S-(2-CARBOXY-3-PHENYLPROPYL)THIODIIMINE-S-METHANE | C11 H16 N2 O2 S | 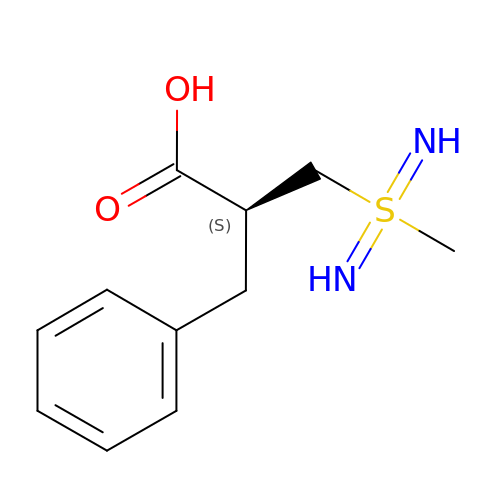FKHYVJWYNYZPCA-SNVBAGLBSA-N> MSNKEKNASETRKAYTTKMIPRSHDRMKLLGNFMDYLMDGTPIFFELWNQFGGGIDRDIISGTANKDKISDDLLLAVNWFKVMPINSKPQGVSPSNLANLFQQYSGSEPDIQAQEYFASNFDTEKHQWKDMRVEYERLLAELQLSRSDMHHDLKLMYKEKCIGLSLSTAHYITSVMFGTGAKNNRQTKHQFYSKVIQLLEESTQINSVEQLASIILKAGDCDSYRKLRIRCSRKGATPSILKIVQDYELGTNHDDEVNVPSLIANLKEKLGRFEYECEWKCMEKIKAFLASKVGPYYLGSYSAMLENALSPIKGMTTKNCKFVLKQIDAKNDIKYENEPFGKIVEGFFDSPYFESDTNVKWVLHPHHIGESNIKTLWEDLNAIHSKYEEDIASLSEDKKEKRIKVYQGDVCQTINTYCEEVGKEAKTPLVQLLRYLYSRKDDIAVDKIIDGITFLSKKHKVEKQKINPVIQKYPSFNFGNNSKLLGKIISPKDKLKHNLKCNRNQVDNYIWIEIKVLNTKTMRWEKHHYALSSTRFLEEVYYPATSENPPDALAARFRTKTNGYEGKPALSAEQIEQIRSAPVGLRKVKKRQMRLEAARQQNLLPRYTWGKDFNINICKRGNNFEVTLATKVKKKKEKNYKVVLGYAANIVRKNTYAAIEAHANGDGVIDYNDLPVKPIESGFVTVESQVRDKSYDQLSYNGVKLLYCKPHVESRRSFLEKYRNGTMKDNRGNNIQIDFMKDFEAIADDETSLYYFNMKYCKLLQSSIRNHSSQAKEYREEIFELLRDGKLSVLKLSSLSNLSFVMFKVAKSLIGTYFGHLLKKPKNSKSDVKAPPITDEDKQKADPEMFALRLALEEKRLNKVKSKKEVIANKIVAKALELRDKYGPVLIKGENISDTTKKGKKSSTNSFLMDWLARGVANKVKEMVMMHQGLEFVEVNPNFTSHQDPFVHKNPENTFRARYSRCTPSELTEKNRKEILSFLSDKPSKRPTNAYYNEGAMAFLATYGLKKNDVLG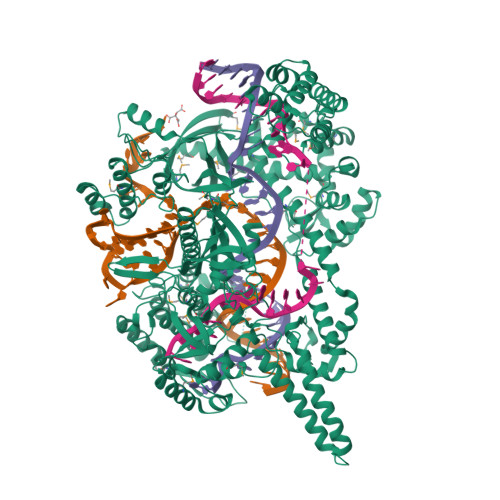VSLEKFKQIMANILHQRSEDQLLFPSRGGMFYLATYKLDADATSVNWNGKQFWVCNADLVAAYNVGLVDIQKDFKKKLEHHHHHH> MGVVREAIAYFAKEAGALSEAELE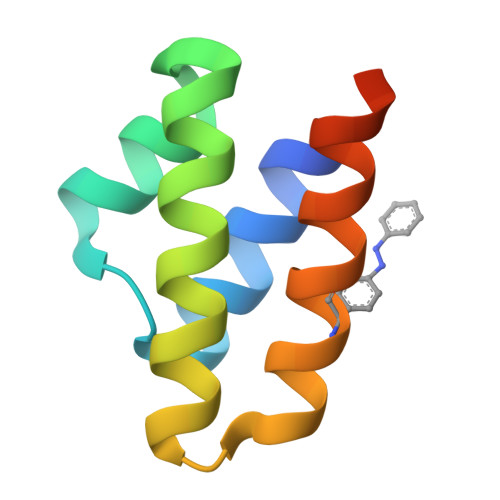KVKNGSNEEAIALGEKAVARAKALGKEKEAKFIKVLVEELKKEGHHHHHH>[2x]MSEMTPREIVSELDKHIIGQDNAKRSVAIALRNRWRRMQLNEELRHEVTPKNI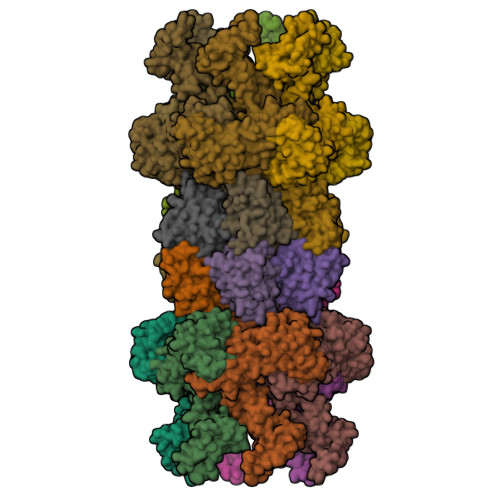LMIGPTGVGKTEIARRLAKLANAPFIKVEATKFTEVGYVGKEVDSIIRDLTDAAVKMVRVQAIEKNRYRAEELAEERILDVLIPPAKNNWGQTEQQQEPSAARQAFRKKLREGQLDDKEIEIDLAAAPMGVEIMAPPGMEEMTSQLQSMFQNLGGQKQKARKLKIKDAMKLLIEEEAAKLVNPEELKQDAIDAVEQHGIVFIDEIDKICKRGESSGPDVSREGVQRDLLPLVEGCTVSTKHGMVKTDHILFIASGAFQIAKPSDLIPELQGRLPIRVELQALTTSDFERILTEPNASITVQYKALMATEGVNIEFTDSGIKRIAEAAWQVNESTENIGARRLHTVLERLMEEISYDASDLSGQNITIDADYVSKHLDALVADEDLSRFIL;>MSSFHATTIFAVQHKGRSAMSGDGQVTFGQAVVMKHTARKVRKLFNGKVLAGFAGSVADAFTLFEKFEAKLEEYNGNLKRAAVELAKEWRSDKVLRKLEAMLIVMNQDTLLLVSGTGEVIEPDDGILAIGSGGNYALAAGRALKKHAGESMSASEIARAALETAGEICVYTNDQIILEELE[2x]>SNAMIIRPEQHWFLRLFDAHGSVLSKIIFRLLLNVLMSIIAIISYQWYEQLGIHLTVAPFSLLGIAIAIFLGFRNSASYSRFVEARNLWGTVLIAERTLVRQLRNILPAEHDAHRRIVSYLVAFSWSLKHQLRKTDPTADLRRLLPEERVTEILASSMPTNRILLLAGNEIGQLREAGKLSDITYGLMDNKLDELAHVLGGCERLATTPVPFAYTLILQRTVYLFCTLLPFALVGDLHYMTPFVSVFISYTFLSWDSLAEELEDPFGTAANDLPLNAM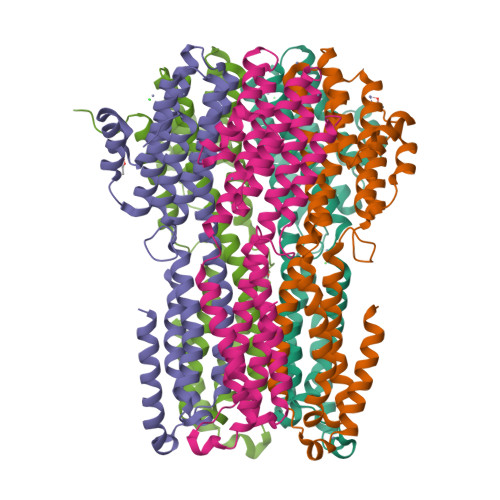CNTIERNLLDMTGQHPLPE[5x]2-[4-(morpholin-4-yl)-6-oxo-1,6-dihydropyrimidin-2-yl]-N-phenylacetamide 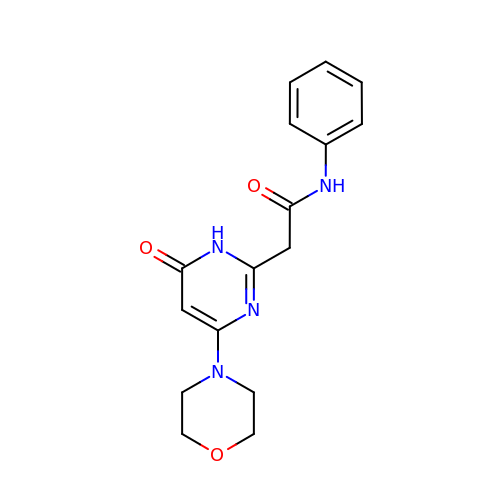| C16 H18 N4 O3 | FPFCFOIMTFHSNY-UHFFFAOYSA-N> MQAEKLGSEIKKIRVLRGLTQKQLSENICHQSEVSRIESGAVYPSMDILQGIAAKLQIPIIHFYEVLIYSDIERKKQFKDQVIMLCKQKRYKEIYNKVWNELKKEEYHPEFQQFLQWQY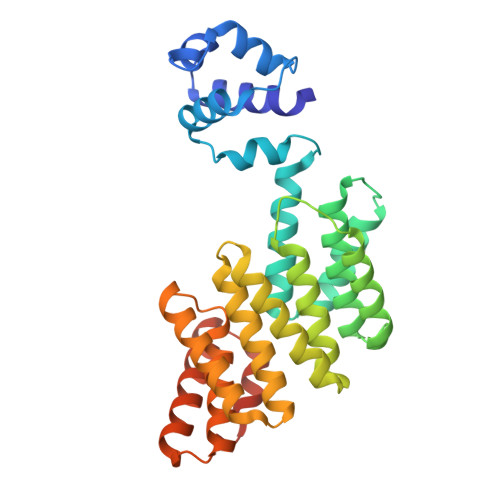YVAAYVLKKVDYEYCILELKKLLNQQLTGIDVYQNLYIENAIANIYAENGYLKKGIDLFEQILKQLEALHDNEEFDVKVRYNHAKALYLDSRYEESLYQVNKAIEISCRINSMALIGQLYYQRGECLRKLEYEEAEIEDAYKKASFFFDILEMHAYKEALVNKISRLEHHHHHH>SMAQRKKYSVYGSCQAPALAKMLNSCPTFARDWELVEMEPCFVASEEQIDRHLAETIPKLDLFLYQPVSEGYRGEKYSSVFLRNSMPPGGNALSVQYMHWEGYHPTVNSPYGLPPHPEGYVDALIAGAVVMDVDKETYLRHLEEIGASLRIDIDEIESWCVDELKTREVGENDGGKQIDISVTDFILANCRQKRLFYTMNHPTAALMREIAARCMLALGYTYSDISFDQNLDPLDVTKMSLYPIYRDCFDFSELNRMNEYQVLYKKKAYEPYLLEQFEWFERSPKADVSAFFDRVAANRRWVRTALRRAFES[2x]

The principal CPS of the human pathogen and Tier 1 select agent Burkholderia pseudomallei consists of a linear repeat of –­3)-­2-O-acetyl-6-deoxy-β-d-manno-heptopyranose-(1–. This CPS is critical to the virulence of this emerging pathogen and represents a key target for the development of novel therapeutics. wcbI is one of several genes in the CPS biosynthetic cluster whose deletion leads to significant attenuation of the pathogen; unlike most others, it has no homologues of known function and no detectable sequence similarity to any protein with an extant structure. The structure revealed that WcbI adopts a predominantly helical fold: the N-terminal 100 amino acids form a ligand-binding domain fold, with the remaining 210 amino acids adopting an entirely novel fold. Based on the structure and on biochemical and biophysical data, we propose that WcbI functions as an acetyltransferase and requires another functional module to carry out this function.

Here, the crystal structure of WcbI bound to its proposed product, coenzyme A, is reported at 1.38 Å resolution, solved using the halide-soak method with multiple anomalous dispersion. Analysis of early crystals of WcbI revealed that an unidentified ligand had been partially retained with the protein from expression in E. coli through the purification process. We therefore co-crystallized WcbI with acetyl-CoA. A second crystal was obtained co-crystallized with substrate acetyl-CoA, and high-resolution complex data were collected. The structure of the CoA complex of WcbI and the native structure were refined by PHENIX and CCP4, respectively, to resolutions of 1.38 and 1.56 Å, respectively. Co-crystallization with 200 µM acetyl-CoA led to almost complete occupancy of the ligand, with all CoA ligand atoms visible in the density. Although there is low occupancy of the acetyl group in the structure, the functional groups of acetyl-CoA form an extensive set of interactions with the protein, supporting the premise that this is a bona fide ligand of WcbI. Furthermore, the acetyl moiety is held in place through hydrogen bonds to Cys14 and His201, constraining its conformation and presenting the acetyl group in a suitable orientation for reaction. Soaks with acetyl-CoA reveal that the CoA head, and likely the acetyl group, are held between cysteine and histidine side chains from opposite sides of the cradle in a conformation suggestive for reaction. The two structures of WcbI presented here, obtained under different conditions, suggest that WcbI allows some flexibility in the CoA head group.> MNITVELTFFEPYRLVEWFDWDARKKSHSAMRGQAFAQWTWKGKGRTAGKSFITGTLVRSAVIKAVEELLSLNNGKWEGVPCCNGSFQTDESKGKKPSFLRKRHTLQWQANNKNICDKEEACPFCILLGRFDNAGKVHERNKDYDIHFSNFDLDHKQEKNDLRLVDIASGRILNRVDFDTGKAKDYFRTWEADYETYGTYTGRITLRNEHAKKLLLASLGFVDKLCGALCRIEVIKKSESPLPSDTKEQSYTKDDTVEVLSEDHNDELRKQAEVIVEAFKQN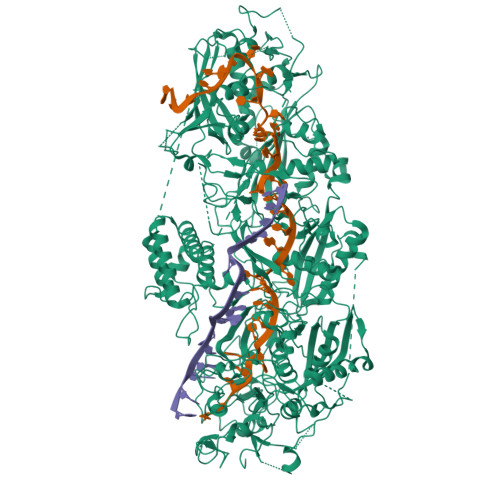DKLEKIRILADAIRTLRLHGEGVIEKDELPDGKEERDKGHHLWDIKVQGTALRTKLKELWQSNKDIGWRKFTEMLGSNLYLIYKKETGGVSTRFRILGDTEYYSKAHDSEGSDLFIPVTPPEGIETKEWIIVGRLKAATPFYFGVQQPSDSIPGKEKKSEDSLVINEHASFNILLDKENRYRIPRSALRGALRRDLRTAFGSGCNVSLGGQILCNCKVCIEMRRITLKDSVSDFSEPPEIRYRIAKNPGTATVEDGSLFDIEVGPEGLTFPFVLRYRGHKFPEQLSSVIRYWEENDGKNGMAWLGGLDSTGKGRFALKDIKIFEWDLNQKINEYIKERGMRGKEKELLEMGESSLPDGLIPYKFFEERECLFPYKENLKPQWSEVQYTIEVGSPLLTADTISALTEPGNRAAIAYKKRVYNDGNNAIEPEPRFAVKSETHRGIFRTAVGRRTGDLGKEDHEDCTCDMCIIFGNEHESSKIRFEDLELINGNEFEKLEKHIDHVAIDRFTGGALDKAKFDTYPLAGSPKKPLKLKGRFWIKKGFSGDHKLLITTALSDIRDGLYPLGSKGGVGYGWVAGISIDDNVPDDFKEMINKTEMPLPEEVEESNNGPINNDYVHPGHQSPKQDHKNKNIYYPHYFLDSGSKVYREKDIITHEEFTEELLSGKINCKLETLTPLIIPDTSDENGLKLQGNKPGHKNYKFFNINGELMIPGSELRGMLRTHFEALTKSCFAIFGEDSTLSWRMNADEKDYKIDSNSIRKMESQRNPKYRIPDELQKELRNSGNGLFNRLYTSERRFWSDVSNKFENSIDYKREILRCAGRPKNYKGGIIRQRKDSLMAEELKVHRLPLYDNFDIPDSAYKANDHCRKSATCSTSRGCRERFTCGIKVRDKNRVFLNAANNNRQYLNNIKKSNHDLYLQYLKGEKKIRFNSKVITGSERSPIDVIAELNERGRQTGFIKLSGLNNSNKSQGNTGTTFNSGWDRFELNILLDDLETRPSKSDYPRPRLLFTKDQYEYNITKRCERVFEIDKGNKTGYPVDDQIKKNYEDILDSYDGIKDQEVAERFDTFTRGSKLKVGDLVYFHIDGDNKIDSLIPVRISRKCASKTLGGKLDKALHPCTGLSDGLCPGCHLFGTTDYKGRVKFGFAKYENGPEWLITRGNNPERSLTLGVLESPRPAFSIPDDESEIPGRKFYLHHNGWRIIRQKQLEIRETVQPERNVTTEVMDKGNVFSFDVRFENLREWELGLLLQSLDPGKNIAHKLGKGKPYGFGSVKIKIDSLHTFKINSNNDKIKRVPQSDIREYINKGYQKLIEWSGNNSIQKGNVLPQWHVIPHIDKLYKLLWVPFLNDSKLEPDVRYPVLNEESKGYIEGSDYTYKKLGDKDNLPYKTRVKGLTTPWSPWNPFQVIAEHEEQEVNVTGSRPSVTDKIERDGKMV>SENPFIAHELKQTSVNEITAHVINEPASLKLTTISTILHAPLQNLLKPRKHRLRVQVVDFWPKSLTQFAVLSQPPSSYVWMFALLVRDVSNVT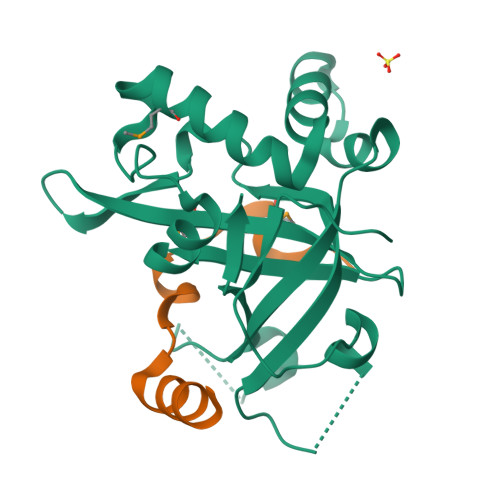LPVIFFDSDAAELINSSKIQPCNLADHPQMTLQLKERLFLIWGNLEERIQHHISKGESPTLAAEDVETPWFDIYVKEYIPVIGNTKDHQSLTFLQKRWRGFGTKIV[2x];>[2x]SQQEKPNDNTSNSRDIKNNIQFHWKNMTSLSIEECIIPKGQQLILEKESEENTTHGIYLEERKMAQGLHNSVSETPE>[2x]MPLCLKINKKHGEQTRRI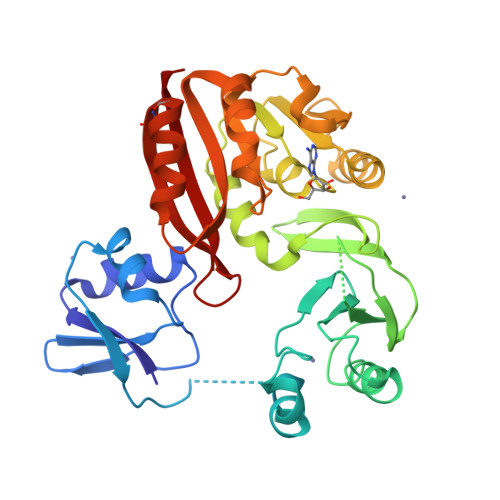LIENNLLNKDYKITSEGNYLYLPIKDVDEDILKSILNIEFELVDKELEEKKIIKKPSFREIISKKYRKEIDEGLISLSYDVVGDLVILQISDEVDEKIRKEIGELAYKLIPCKGVFRRKSEVKGEFRVRELEHLAGENRTLTIHKENGYRLWVDIAKVYFSPRLGGERARIMKKVSLNDVVVDMFAGVGPFSIACKNAKKIYAIDINPHAIELLKKNIKLNKLEHKIIPILSDVREVDVKGNRVIMNLPKFAHKFIDKALDIVEEGGVIHYYTIGKDFDKAIKLFEKKCDCEVLEKRIVKSYAPREYILALDFKINKK>MSDAAPSLSNLFYDPTYNPGQSTINYTSIYGNGSTITFDELQGLVNSTVTQAIMFGVRCGAAALTLIVMWMTSRSRKTPIFIINQVSLFLIILHSALYFKYLLSNYSSVTYALTGFPQFISRGDVHVYGATNIIQVLLVASIETSLVFQIKVIFTGDNFKRIGLMLTSISFTLGIATVTMYFVSAVKGMIVTYNDVSATQDKYFNASTILLASSINFMSFVLVVKLILAIRSRRFLGLKQFDSFHILLIMSCQSLLVPSIIFILAYSLKPNQGTDVLTTVATLLAVLSLPLSSMWATAANNASKTNTITSDFTTSTDRFYPGTLSSFQTDSINNDAKSSLRSRLYDLYP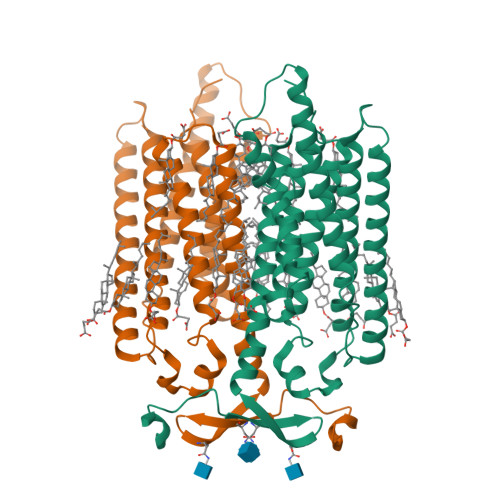RRKETTSDKHSERTFVSETADDIEKNQFYQLPTPTSSKNTRIGPFADASYKEGEVEPVDMYTPDTAADEEARKFWTEDNNNL[2x]>SNALLTGKKILVVDDNIVNRRVAAGALKKFGAEVVCAESGQVALGLLQIPHTFDACFMDIQMPQMDGFEATRQIRMMEKETKEKTNLEWHLPILAMTADVIHATYEECLKSGMDGYVSKPFEEENLYKSVAKSFKPNPISPSS[2x]

CYTOKININ RESPONSE1 (CRE1), the main cytokinin receptor, has a modular architecture composed of a cytokinin-binding CHASE (Cyclases/Histidine kinases Associated Sensory Extracellular) domain, followed by a transmembrane fragment, an intracellular histidine kinase (HK) domain, and a receiver domain (REC). Perception of cytokinin signaling involves (i) a hormone molecule binding to the CHASE domain, (ii) CRE1 autophosphorylation at a conserved His residue in the HK domain, followed by a phosphorelay to (iii) a conserved Asp residue in the REC domain, (iv) a histidine-containing phosphotransfer protein (HPt), and (v) a response regulator (RR). This work focuses on the crystal structures of the REC domain of CRE1 from the model plant Arabidopsis thaliana and from the model legume Medicago truncatula.

The structure of AtCRE1-REC was determined in two isomorphous variants of space group P21212 with two protein subunits (chains A and B) in the asymmetric unit forming a homodimer. The structure of the AtCRE1-REC-Mg2+ complex (referred to as AtCRE1-REC-Mg), determined at 1.7 Å resolution, encompasses residues Leu918-Ser1057, extended at the N-terminus by a Ser-Asn-Ala cloning artifact. In the final model, subunit A is comprised of 139 residues and subunit B of 127 residues. In chains A and B, there are two, and 15 missing residues (Ser1056-Ser1057/Ser1043-Ser1057), respectively, which could not be modeled in the electron density because of disorder. Each subunit binds a magnesium cation. There are 182 water molecules, one ethylene glycol and one (4S)-2-methyl-2,4-pentadiol (MPD) molecule in the asymmetric unit. For protein structure analysis, the full C-terminal construct from the Mg2+ complex above is used. In the AtCRE1-REC-Mg complex, the octahedral coordination sphere consists of six oxygen atoms: two Oδ of Asp929 and Asp973, one backbone O atom of Gln975 and three water molecules. The lengths of the Mg-O coordination bonds range from 2.15 to 2.30 Å. As a result, the Mg2+ ion lies farther away from Asp1013 and a water molecule fills up the coordination sphere, bridging it with the Oδ atom of Asp1013 (helix α4).> ARSTNTFNYATYHTLDEIYDFMDLLVAEHPQLVSKLQIGRSYEGRPIYVLKFSTGGSNRPAIWIDLGIHSREWITQATGVWFAKKFTEDYGQDPSFTAILDSMDIFLEIVTNPDGFAFTHSQNRLWRKTRSVTSSSLCVGVDANRNWDAGFGKAGASSSPCSETYHGKYANSEVEVKSIVDFVKDHGNFKAFLSIHSYSQLLLYPYGYTTQSIPDKTELNQVAKSAVAALKSLYGTSYKYGSIITTIYQASGGSIDWSYNQGIKYSFTFELRDTGRYGFLLPASQIIPTAQETWLGVLTIMEH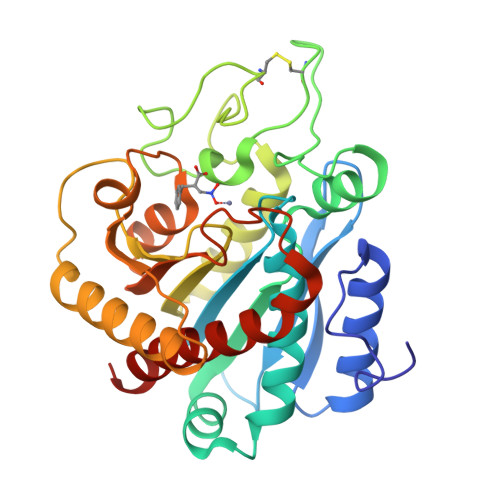TVNN> AM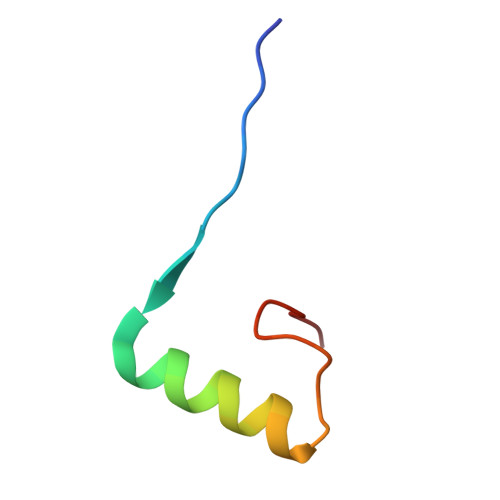AAKVVYVFSTEMANKAAEAVLKGQVETIVSFHI> DEEEIQKAIEELLRKGVSEEEAAIIIVQRFNVAVVVVVQDERQAKHISEYIRRYIPEADVILFANIVVIKVETHELRK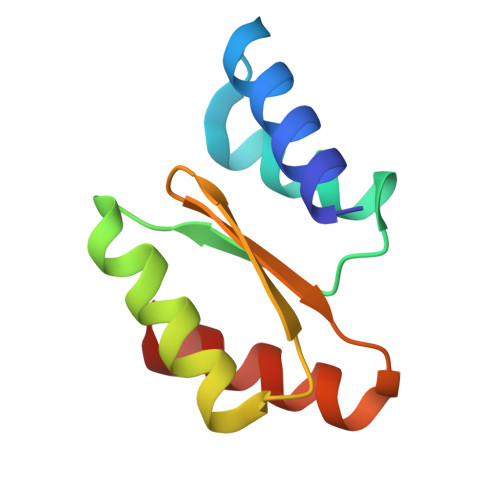RVWEAAQKAY>GHMASMAKIKNQYYNESVSPIEYAQQGFKGKMRSVNWNVVNDEKDLEVWNRITQNFWLPEKIPVSNDLTSWRTLTPEWQELITRTFTGLTLLDTIQATVGDVAQVPNSLTDHEQVIYTNFAFMVAVHARSYGSIFSTLCSSEQIEEAHEWVINTETLQERAKALIPYYVNDDPLKSKVAAALMPGFLLYGGFYLPFYLSARGKLPNTSDIIRLILRDKVIHNYYSGYKYQKKVAKLSPEKQAEMKEFVFKLLYELIDLEKAYLKELYEDFGLADDAIRFSVYNAGKFLQNLGYDSPFTEEETRI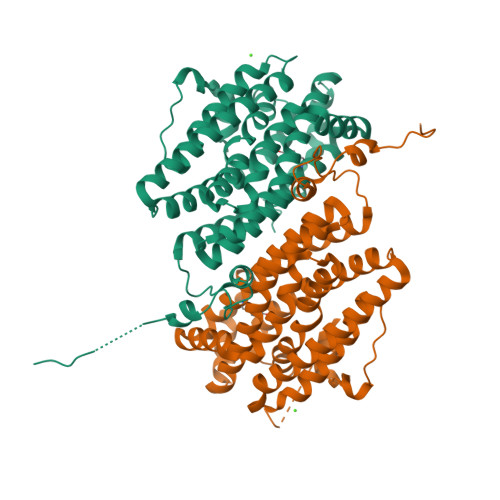EPEIFTQLSARADENHDFFSGNGSSYIMGVSEETEDDDWEF[2x]>[2x]MTSKVYDPEQRKRMITGPQWWARCKQMNVLDSFINYYDSEKHAENAVIFLHGNATSSYLWRHVVPHIEPVARCIIPDLIGMGKSGKSGNGSYRLLDHYKYLTAWFELLNLPKKIIFVGHDFGAALAFHYAYEHQDRIKAIVHMQSVVDVIESWDEWPDIEEDIALIKSEEGEKMVLENNFFVETVLPSKIMRKLEPEEFAAYLEPFKEKGEVRRPTLSWPREIPLVKGGKPDVVQIVRNYNAYLRASDDLPKLFIESDPGFFSNAIVEGAKKFPNTEFVKVKGLHFLQEDAPDEMGKYIKSFVERVLKNEQHHHHHH

The light-producing reaction catalysed by the Renilla-type luciferase is one of the most widely used biochemical reactions in molecular and cell biology research. Here we track the role of dynamics in evolution, starting from the evolvable and thermostable ancestral protein AncHLD-RLuc which catalyses both dehalogenase and luciferase reactions. The regions encompassing the L9-α4 fragment and L14 loop are important structural elements that line the main access tunnels connecting the buried active site to the surrounding solvent. We conclude that the LUC activity benefits from conformational dynamics of the protein’s rigid scaffold to allow binding of a bulky substrate.

To ascertain the role of the L9-α4 fragment in substrate binding, we tried to co-crystallize RLuc8 with CTZ. In contrast, mixing the RLuc8-W121F/E144Q mutant with CTZ yielded a high-resolution complex structure with coelenteramide (CEI), which is the product of the LUC reaction. Unlike in an RLuc8-CEI complex structure, the CEI molecule in our complex is inverted by nearly 180°, which allows its accommodation in the luciferase active site cavity. The rest of the CEI molecule occupies the main enzyme access tunnel, where it is tightly wrapped by multiple, predominantly hydrophobic, residues: V146, I150, I159, V185, F181, F261, F262, H285 and I266. Interestingly, many of the residues directly interacting with the CEI are located on the loop L9 (V146, I150, W156 and I159) and the loop L14 (I223 and P224), identified as important for catalysis by our directed evolution experiments. The α4 helix is in an open conformation relative to the α5 helix.> MLGNMNVFMAVLGIILFSGFL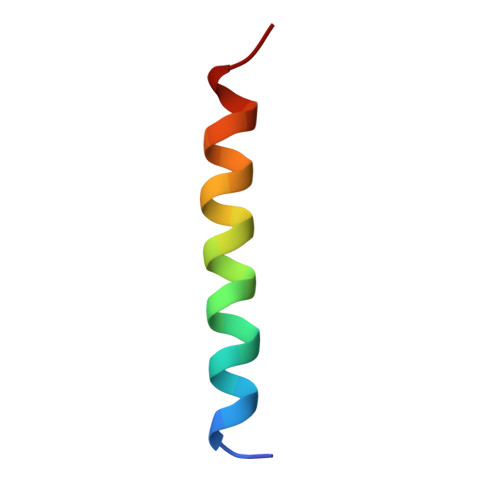AAYFSH>[123x]MTCTTGAGVTSGFIDLATYDNLDRALYGGKDATTYFIKEHYPVGWFTKLPTMATRVSGNPAFGQEFSVGVPRSGDYVLNAWLTLKTPEIKLLETNRLGANGTVRWTKNLMHNAVEHASLTFNDICAQQFNTAYLDAWTQFNMCEGKRIGYDNMIGNTSDMTNPTPAQGQDGARTLPSKNLVLPLPFFFSRDCGLALPTVVLPYNEIRINIKLRSLQELLVFQNKDTGNVIPISATDIAGGLADTVEAYVYMTVGLVSNVERCAMAGTVRDMVVEQMQAAPTHIVNPQNTNNVHVDMRFSHAVKALFFMVQNVTYKSVGSNYTCVTPVNGPGNTVMEPAMSVDPIKSASLTYENTTRLANMGVEYYSLVQPWYFSASIPVYTGYHMYSYALNVGS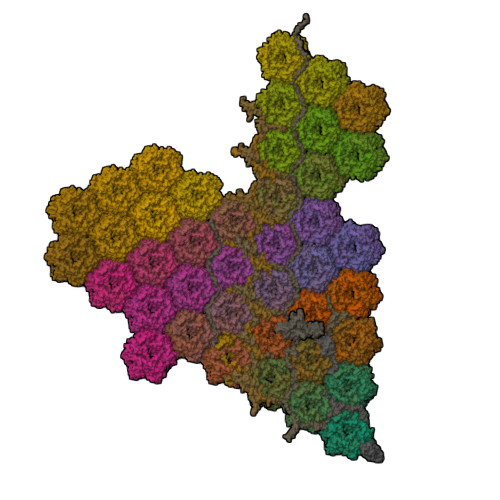VHPSGSTNYGRLTNASITVTMSPESVVAAAGGGNNNSGYNEPQRFALVVIAVNHNVIRIMNGSMGFPIL;>[15x]MIHNYAILIVTAAVVVWYYYKLYVVDKNGKKSLVRTRKHRNLESAARRDPILKTYSKQDGTRSRKPKSTKKEPHWMDPQLMGSQTTQYSRNRGYGDPIRGDLPIVPDDGGWFATRANPAHHLHTGALSMIGGDASDCGSTAVQQLIKKYEDKGCNNNGLNVMSSHYGGVM;>MDCATYATRKDKGWELNENRCVWAASVKPTSGAIMTNVGVHGKSGNAVLMTPKRRPHAQNHAGYKIKYCKQVPLIPLHGGDYILNHWETRGVDRMRIPGIQHAPPPPAPSGMQNAYSTHPDAYRTPLLADSHALSRMPVVQVHGPQVAPKNSHFTVAPEKHGPVEDMNAIINALPTKVDAVKLEYSASKTNRTNKRPGDGGAPPPKNLSKCHQNKLKTFARTANSGANPFRPATAAPQGLSKQPVRKPFASARNANSGANPFRPPLAHQGLSKAHVVKTAVSVANRSAGAEPFVTRNDPRALAMELANNKTISVTLGLRHWKTVSAAPPEKMSKSGVCKIATNVYNRDGGANPFLVKYEPDSLAVCPMETVEIAAVPSKRPWEGSANPRRPEQISFGMSDKPKFVNDKIGIVLRGPTLAPTLDRTATHTVTRPRALGSFHSTAGPAKHAASIMAECKDESR[2x];> MYRGFSLKLPNNYRSGQVTTEHRLPASNSHARWPVEVSFYSAVLHVPAKHQHKFPPVLELKLHNMTTGSMAAHRGSGHHFTFMFHAQSSPTEAVYSCVPVPIVFSDYQSNVIASVDMGEHDTAEKLHFYGSIRNCDNGCTY;> MGAAQSVNGVKIVTNAYAEIMTDLAVDQDITADQTQVFSIDNVSGDVYVEGTVMTEKLVINLASLMKAVTNQSSQDELIDNIAQQAQAAVSGLNFAQFAFVTNNIDRLITACVKLSVDMRVSCTAKVEMTQSFSVSSVMGDVRVKDVRMEEFSDVISTCALNAAITNAQLSDIVSQIKQRGDATATGLNPMAILAAVVLAIIGLPLGAGFLAGRRVVGPLMMVTGMVGGGALAMGYVPEPIKLTGFAPEPDLTAVVPVAVENGLTLKAAISKLTGDPQYGAVYWQNYKVTGTTAVKLNQTVSYYAPPNFDPVTWTASEPAQKQPSFRVFPTLFQGQGLPKISYRLAYGTVALTQGPERGDVYLDSTTGNYYVLKDGWKLNGTIPGAIKDRPEAWGIVDPNETTALTGSERYTWVDPYTRVQGTLWYKPKDSHEWVKERQDPVPINVPLTETPSDFNVWVYKDATAKKIVGWVSAGAGAAGAGLTASAYFMPSTAVDAKAEVGEAAK;> MDSQGFWAILAFTPVLMILSLKGEGLLAMVGLLVLTVTLLASREKNDRPRLSCRGKIGRKVSGFENAGHVRDSHHVIYKRPPVNEYCAETREDNSLYVPEYCGQNWKNGVLSGMGTHHDAYRNLAVNMMTLRRESAVSAGWAHSYL;> MNAYQNDKLHLCAPRPDLVRAAMSAMVRETGCTPNVNIREMAISAGVMLTKIRANPGMLRYGMTATQTVIYNLKELFAAHAARGVVFKTPAIHPAHPSQWKGF> IPPIPPVDFAKYGEIEEVPMTRLMQIGATNLHRSWLNVPHVTQFESADITELEAFRVAQKAVAEKAGVKLTVLPLLLKACAYLLKELPDFNSSLAPSGQALIRKKYVHIGFAVDTPDGLLVPVIRNVDQKSLLQLAAEAAELAEKARSKKLGADAMQGACFTIAS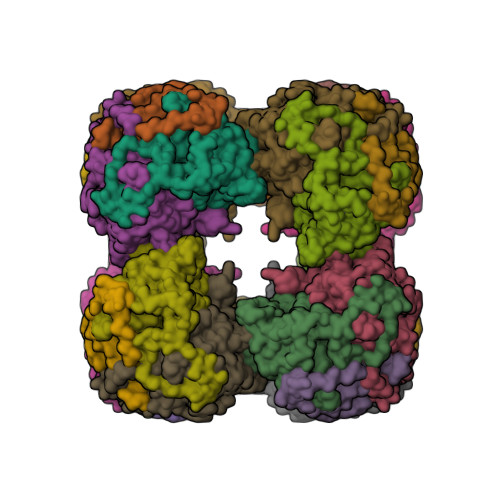LGHIGGTAFTPIVNAPEVAILGVSKASMQPVWDGKAFQPRLMLPLSLSYDHRVINGAAAARFTKRLGDLLADIRAILL>HHHHHHSGMKQLTILGSTGSIGCSTLDVVRHNPEHFRVVALVAGKNVTRMVEQCLEFSPRYAVMDDEASAKLLKTMLQQQGSRTEVLSGQQAACDMAALEDVDQVMAAIVGAAGLLPTLAAIRAGKTILLANKESLVTCGRLFMDAVKQSKAQLLPVDSEHNAIFQSLPQPIQHNLGYADLEQNGVVSILLTGSGGPFRETPLRDLATMTPDQACRHPNWSMGRKISVDSATMMNKGLEYIEARWLFNASASQMEVLIHPQSVI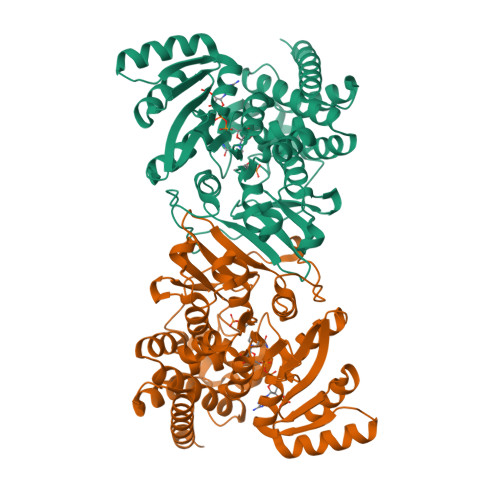HSMVRYQDGSVLAQLGEPDMRTPIAHTMAWPNRVNSGVKPLDFCKLSALTFAAPDYDRYPCLKLAMEAFEQGQAATTALNAANEITVAAFLAQQIRFTDIAALNLSVLEKMDMREPQCVDDVLSVDANAREVARKEVMRLAS[2x]>MALLEICCYSMECALTAQQNGADRVELCAAPKEGGLTPSLGVLKSVRQRVTIPVHPIIRPRGG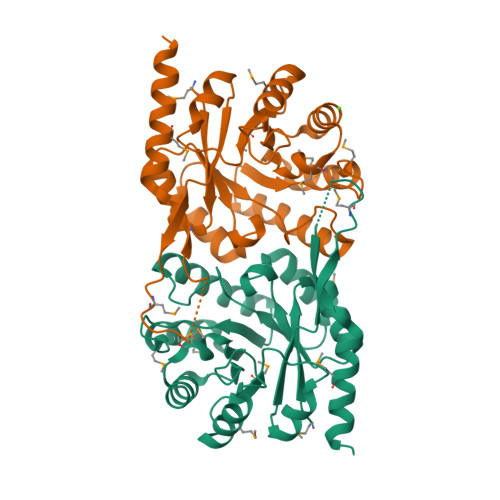DFCYSDGEFAAILEDVRTVRELGFPGLVTGVLDVDGNVDMPRMEKIMAAAGPLAVTFHRAFDMCANPLYTLNNLAELGIARVLTSGQKSDALQGLSKIMELIAHRDAPIIMAGAGVRAENLHHFLDAGVLEVHSSAGAWQASPMRYRNQGLSMSSDEHADEYSRYIVDGAAVAEMKGIIERHQAKLEHHHHHH[2x]>[4x]MSVFVSGANGFIAQHIVDLLLKEDYKVIGSARSQEKAEN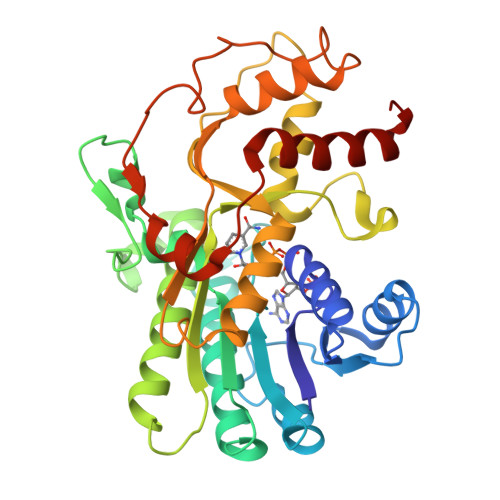LTEAFGNNPKFSMEVVPDISKLDAFDHVFQKHGKDIKIVLHTASPFCFDITDSERDLLIPAVNGVKGILHSIKKYAADSVERVVLTSSYAAVFDMAKENDKSLTFNEESWNPATWESCQSDPVNAYCGSKKFAEKAAWEFLEENRDSVKFELTAVNPVYVFGPQMFDKDVKKHLNTSCELVNSLMHLSPEDKIPELFGGYIDVRDVAKAHLVAFQKRETIGQRLIVSEARFTMQDVLDILNEDFPVLKGNIPVGKPGSGATHNTLGATLDNKKSKKLLGFKFRNLKETIDDTASQILKFEGRI>MGSSHHHHHHENLYFQSNAEQVFQNFETLQLHAGYTPDPHTRSTAVPIYATSSYTFNDSAHGARLFGLKELGNIYSRLMNPTVDVFEKRIAALEGGIAAAATSSGQAAQFLTIATLAKAGDNIVASSHLYGGTYNQLNVLLPRFGIKTKFVRSGKLEDYAAAIDDQTRAIYVESMSNPDYVVPDFEGIAKIAHEHGIPLVVDNTLGAGGYYIRPIEHGADIVVHSATKWIGGHGTTIGGVIVDSGRFNWNKHSDRFPEMVEPSPSYHGLKYWEAFGPATFITRIRVEMLRDIGACLSPFSAQQLLLGIETLGLRAERHAQNTEKLSKYFESSPNVSWVLWPGSESHPTYSQAKKYLTRGFGAMLSIGVK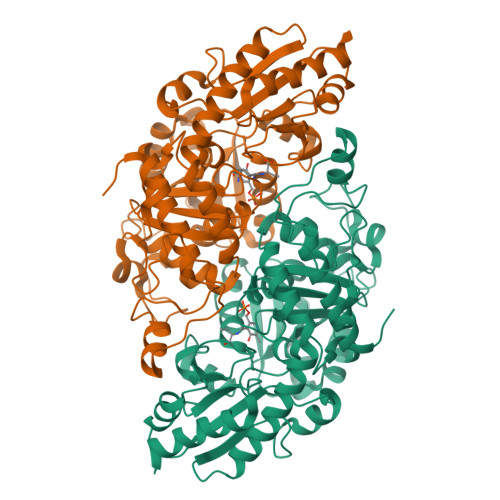GDASAGSKVVDGLKLVSNLANVGDAKSLAIHPWSTTHEQLSEDERLASGVTEDMIRISVGIEHVDDIIADFEQSFQKAYGS[8x]> IELPDAISDGEVRKLVENEFWPEFVRRREKLDRIAQWARGEQPDYLIQNANREKRALLKLAKTPWLGLVVTHFTQALFVDGYRAEGSKENAKGPWQTWNANKMQSKQIAIHRAA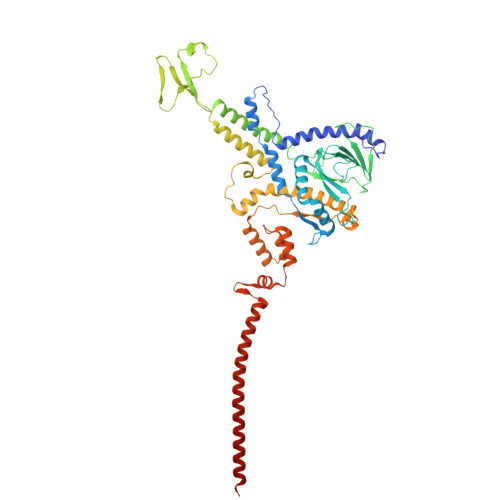LTYGYSYARVLPGVALDGANQAEIHGVSPRRLLALYEDQINDEYPKYALELANNGKTVRLYTDTDYYELRMPSPGNFPNEQVIKKVHHGVGVCPFVRYVNMMDLDGFTMGEVEYLVPVASKIDKTDYDRLLAQHYNSWKVKVATGIDDLSEDATPEEQQRAKLILAQDDILMHGNHEAKFYTLPETSLDGFIAAHTQDVEILANNAQVPVWILNGQLANLSADALTAATKGTIQKLYERQVTFGAAHNQVLRLAAHVEGDTEGARDFTASVSWQDTSVRSLAQAVDAYGKAATMLGMPKEFLWGLIPGITKTDVEAMRQHFNDDDEMTQMLLWWTPNGPGGEFAAEIEVDSQTQIIEAQGDVQKDLQDAQAKAQADLAKQNAAAQQRQAVAV>[2x]MKLKSFGVFGNPIKHSKSPLIHNACFLTFQKELRFLGHYHPILLPLESHIKSEFLHLGLSGANVTLPFKERAFQVCDKIKGIALECGAVNTLVLENDELVGYNTDALGFYL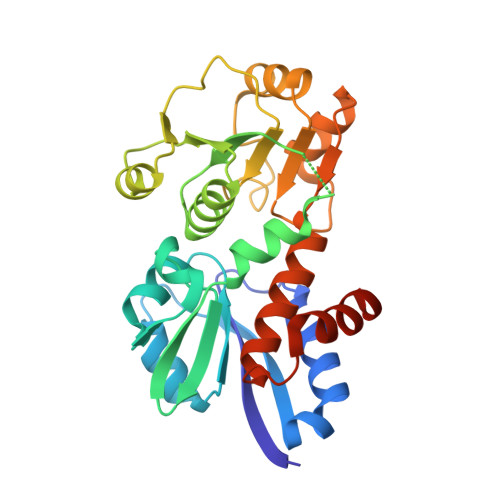SLKQKNYQNALILGAGGSAKALACELKKQGLQVSVLNRSSRGLDFFQRLGCDCFMEPPKSAFDLIINATSASLHNELPLNKEVLKGYFKEGKLAYDLAYGFLTPFLSLAKELKTPFQDGKDMLIYKAALSFEKFSASQIPYSKAFEVMRSVFLEHHHHHH>MEQTQKLKLNLQHFASNNVKPQVFNPDNVMMHEKKDGTLMNEFTTPILQEVMENSKIMQLGKYEPMEGTEKKFTFWADKPGAYWVGEGQKIETSKATWVNATMRAFKLGVILPVTKEFLNYTYSQFFEEMKPMIAEAFYKKFDEAGILNQGNNPFGKSIAQSIEKTNKVIKGDFTQDNIIDLEALLEDDELEANAFISKTQNRSLLRKIVDPETKERIYDRNSDSLDGLPVVNLKSSNLKRGELITGDFDKLIYGIPQLIEYKIDETAQLSTVKNEDGTPVNLFEQDMVALR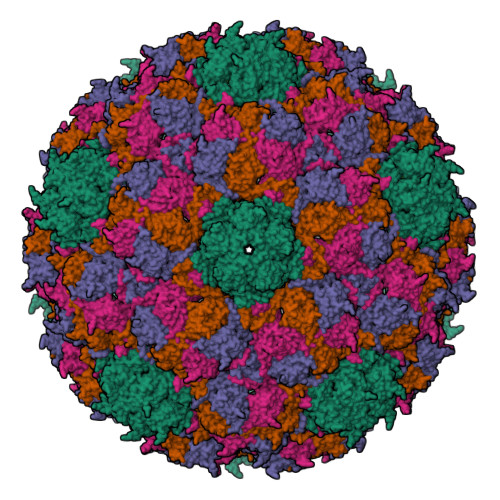ATMHVALHIADDKAFAKLVPADKRTDSVPGEV[4x];>METKYELNNTKKVANAFGLNEEDTNLLINAVDLDIKNNMQEISSELQQSEQSKQKQYGTTLQNLAKQNRIIK[4x]> MVEVKKHKFPGVYTVIDDDGSERIATKNLVPGQRVYGERVIKWEGEEYRIWNPNRSKLGAAIMNGLKNFPIKPGKSVLYLGIASGTTASHVSDIVGWEGKIFGIEFSPRVLRELVPIVEERRNIVPILGDATKPEEYRALVPKVDVIFEDVAQPTQAKILIDNAEVYLKRGGYGMIAVK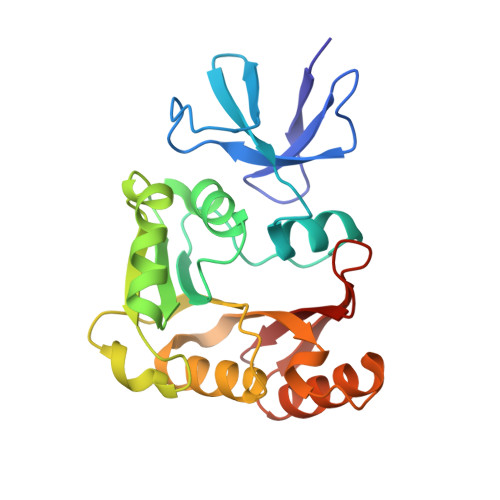SRSIDVTKEPEQVFREVERELSEYFEVIERLNLEPYEKDHALFVVRKT>GALTTSTRQGSRVVGFMDFIIALGWQIIPSNIRYIYILNCSQFMPTSDVTTIYFQADSGLESIFVMDSPFYASCTQQLPDKTIKTYGVTISKKQSIISINFSSSLEPNIMVSAWTASITRTQ[3x]

In adenoviruses, primary host cell recognition is generally performed by the head domains of their homo-trimeric fibre proteins. Cell recognition and attachment are usually initiated by the fibre protein, via its C-terminal head domain. Like other adenovirus fibres, it is predicted to consist of three domains: an N-terminal penton-base binding domain, a shaft domain and a C-terminal fibre head domain. BAdV-4 contains a single fibre gene, encoding a protein of 535 amino acids in length with low sequence identity to known adenovirus fibres (15–19 %).

Here, we report the expression, purification, crystallization and structure solution of the fibre head domain of BAdV-4 at 1.2 Å (0.12 nm) resolution. It is the second atadenovirus fibre head structure that has been solved, after that of the SnAdV-1 fibre head domain; and the first of an atadenovirus which infects mammalian cells. Crystals appeared after three days and grew to their maximal size in about three weeks. They were found to belong to space group P1, with one protein trimer in the unit cell, leading to a solvent content of 44 % and a Matthews coefficient of 2.2. The final refined model contains residues 420–534 from each of the three protein chains in the trimer, plus ordered solvent atoms. The structure of the BAdV-4 fibre head domain is composed of three monomers, associated into a compact trimer. Each monomer consists of a beta-sandwich of two beta-sheets (ABCJ- and GHID-sheets), in the same topology as other adenovirus fibre heads (the topology of the HAdV-5 fibre head is shown as an example in Fig. 3d). The loop between strands D and G is longer than the others and contains an alpha helix (residues 471–476), instead of the E- and F-strands that many mastadenovirus fibre head domains have in this loop. The CD- and IJ-loops run parallel to each other and contain negatively charged residues, forming electronegative patches on the protein surface. The BAdV-4 fibre head shares only 15 % sequence identity with the other atadenovirus fibre head (from SnAdV-1) for which a structure is known. No salt bridges are formed upon trimeric assembly for the BAdV-4 fibre head, while in the SnAdV-1 fibre head a strong bidentate salt bridge between Arg304 and Glu333 of neighbouring monomers is present, which may explain why the SnAdV-1 fibre head is more stable than the BAdV-4 fibre head.>[3x]MEKTCIDALPLTMNSSEKQETVCIFGTGDFGRSLGLKMLQCGYSVVFGSRNPQKTTLLPSGAEVLSYSEAAKKSGIIIIAIHREHYDFLTELTEVLNGKILVDISNNLKINQYPESNAEY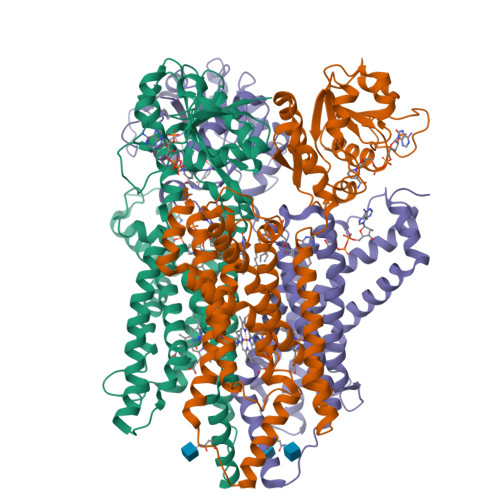LAHLVPGAHVVKAFNTISAWALQSGALDASRQVFVCGNDSKAKQRVMDIVRNLGLTPMDQGSLMAAKEIEKYPLQLFPMWRFPFYLSAVLCVFLFFYCVIRDVIYPYVYEKKDNTFRMAISIPNRIFPITALTLLALVYLPGVIAAILQLYRGTKYRRFPDWLDHWMLCRKQLGLVALGFAFLHVLYTLVIPIRYYVRWRLGNLTVTQAILKKENPFSTSSAWLSDSYVALGILGFFLFVLLGITSLPSVSNAVNWREFRFVQSKLGYLTLILCTAHTLVYGGKRFLSPSNLRWYLPAAYVLGLIIPCTVLVIKFVLIMPCVDNTLTRIRQGWERNSKH6-[(7-methyl-2-propyl-imidazo[4,5-b]pyridin-4-yl)methyl]-2-[2-(1H-1,2,3,4-tetrazol-5-yl)phenyl]-1,3-benzothiazole | C25 H22 N8 S | 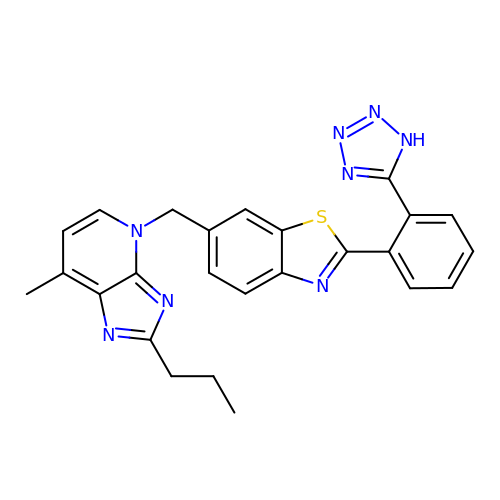LGDMZWWVVLGYPR-UHFFFAOYSA-N1-deoxy-alpha-L-xylulofuranose-1,2-borate | C5 H10 B O6 | 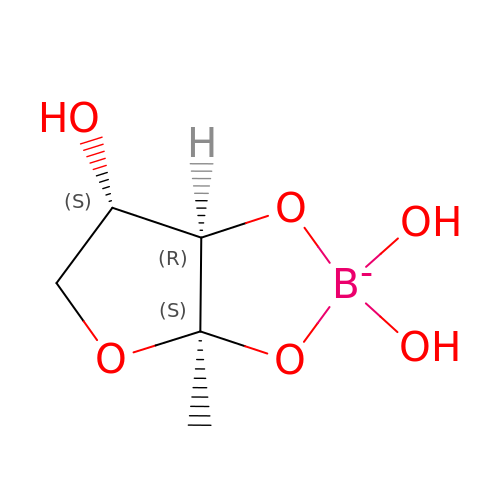GNABZUZRGYHKDZ-VPENINKCSA-N5-(4-morpholin-4-yl-7H-pyrrolo[2,3-d]pyrimidin-5-yl)-2-oxidanyl-benzaldehyde 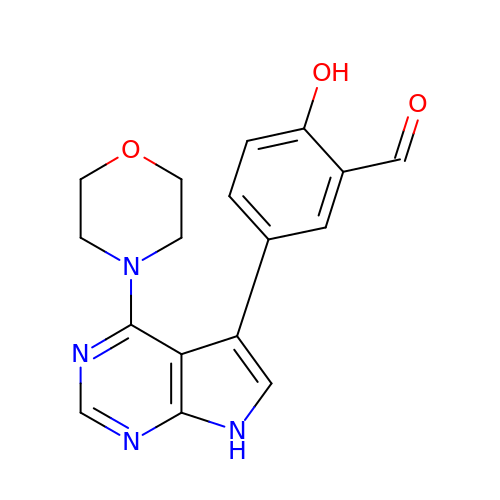| C17 H16 N4 O3 | OPQSSAIBYNXUAR-UHFFFAOYSA-N>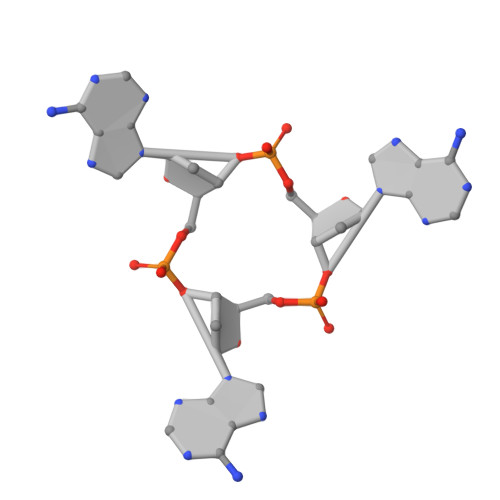[2x]AAA> GPHMTQPLVGKQILIVEDEQVFRSLLDSWFSSLGATTVLAADGVDALELLGGFTPDLMICDIAMPRMNGLKLLEHIRNRG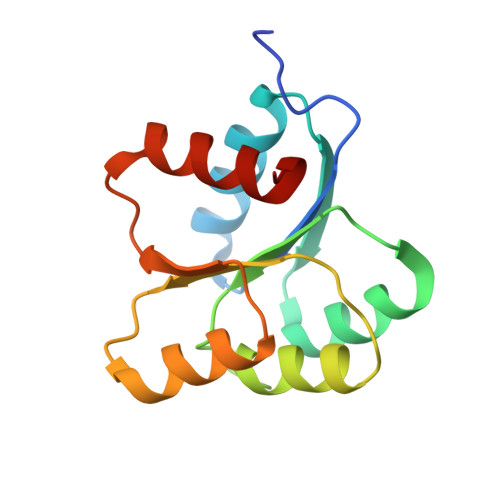DQTPVLVISATENMADIAKALRLGVEDVLLKPVKDLNRLREMVFACLYPSMF>[2x]QI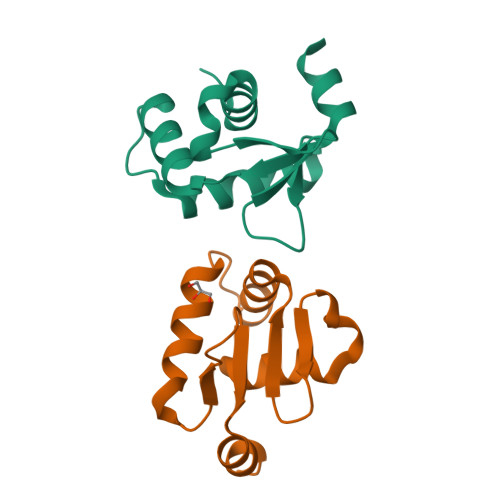QLWQFLLELLSDSSNSSCITWEGTNGEFKMTDPDEVARRWGERKSKPNMNYDKLSRALRYYYDKNIMTKVHGKRYAYKFDFHGIAQALQP>[4x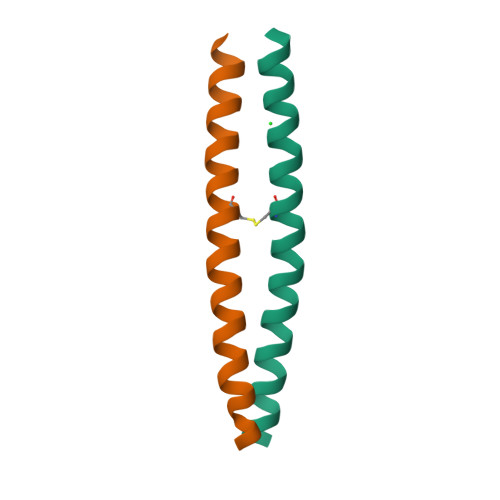]GPLGSKTRSERQLLRLKQMNVQLAAKIQHLEFSCSEKEQEIERLNKLLRQHGLLGEVN>[2x]HSPEEQKQMLGEAIYPKVAASQPELAGKLTGMILELPVTELLHLLEESEALDAK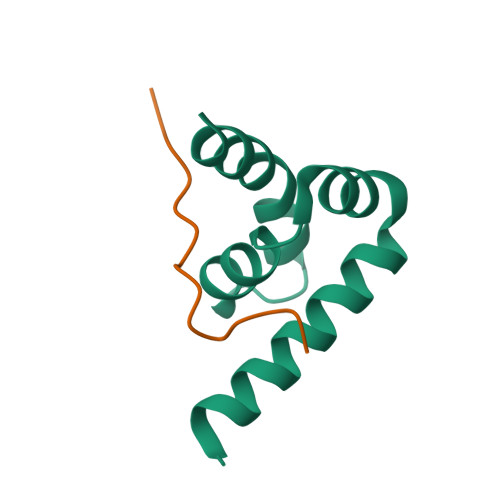VNEALEVLKEYQQN;>[2x]STLSPNASVFKPSRS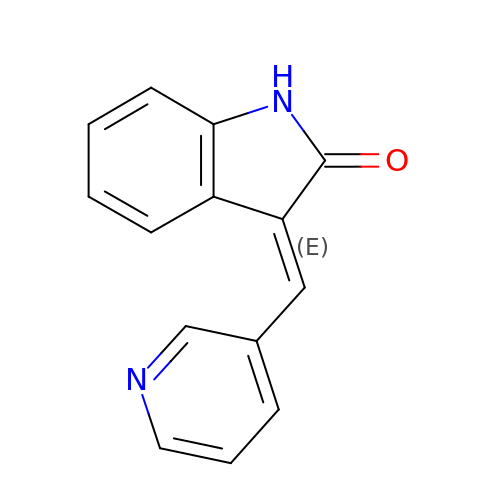(3E)-3-(pyridin-3-ylmethylidene)-1,3-dihydro-2H-indol-2-one | C14 H10 N2 O | ALVGMCFQOGIUFY-XYOKQWHBSA-N> KDGDQCETSPC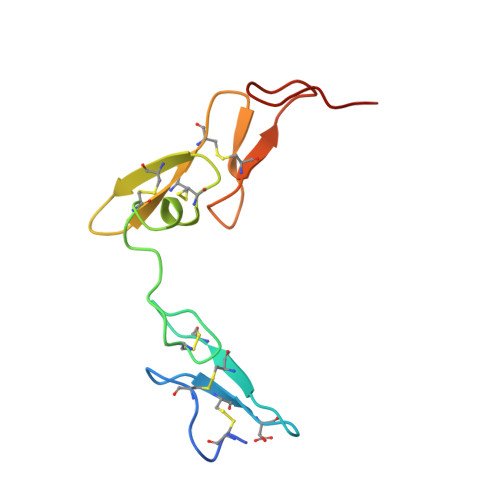QNQGKCKDGLGEYTCTCLEGFEGKNCELFTRKLCSLDNGDCDQFCHEEQNSVVCSCARGYTLADNGKACIPTGPYPCGKQTLER(3~{S},5~{R},6~{R})-5-[(3~{S},7~{R},12~{S},16~{S},20~{S})-3,7,12,16,20,24-hexamethyl-24-oxidanyl-pentacosyl]-4,4,6-trimethyl-cyclohexane-1,3-diol | C40 H80 O3 | 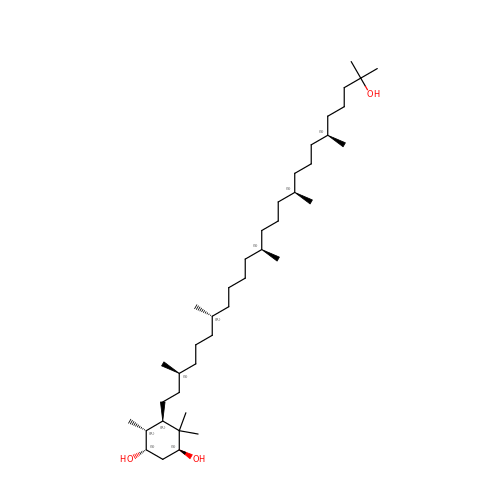HMWJPEUVPLHAER-VMKFVPKQSA-N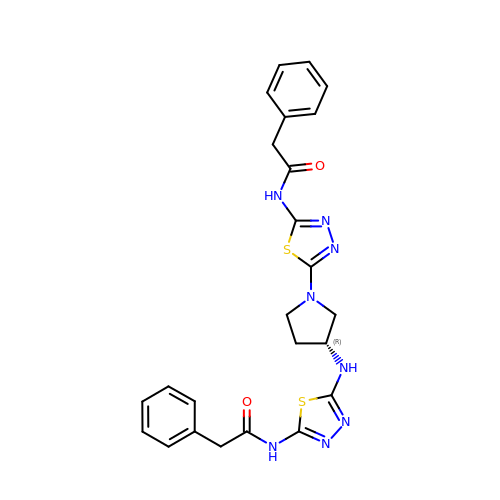2-phenyl-~{N}-[5-[[(3~{R})-1-[5-(2-phenylethanoylamino)-1,3,4-thiadiazol-2-yl]pyrrolidin-3-yl]amino]-1,3,4-thiadiazol-2-yl]ethanamide | C24 H24 N8 O2 S2 | XKAUHJUBYCZSGD-GOSISDBHSA-N>GPLGSMRKQALHPRTAVINKAQKNQSKRARSDALLWLAANFPEAFDNSLRIRPLKIGIMSD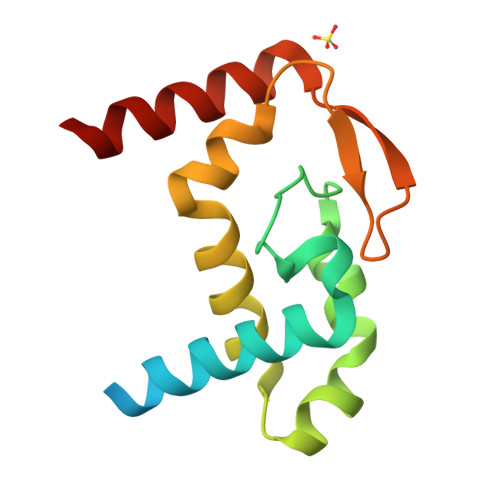ILQHAEKAEQVGVSKSKLREAVVLFTRRLDYLACLKAREVRIDLHGNPVAEVTEEEAENASMKIKKRVEK[9x]>GANAYLNLYKIDIPKKIKRLYFYNPDMEPKLFARNLSRVNNFKFQDSNDLVWIEIPDIDFQITPKNVFQYKVEKEEIIKEEEDKKLFVKTLYKYIKKLFLDNDFYF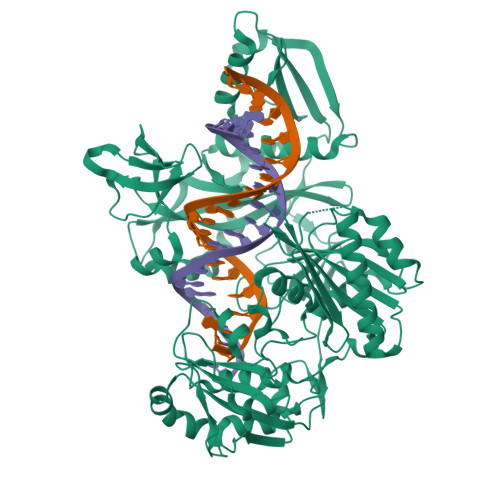KKGNNFISNSEVFSLDSNENVNAHLTYKIKIHNISNEYYLSILPKFTFLSKEPALESAIKSGYLYNIKSGKSFPYISGLDGILKIDIGNNQIVEVAYPENYLFNFTTRDAEKYGFSKEVHEIYKNKVFEGFKKIPKTLGFLNKITNLNENYQLKDGYKIFINVIYKFKNGESRYAKDVFKYSFYKNEQPLKAIFFFSSKKQFFEVQKSLKELFHNKHSVFYRAAAELGFSKVEFLRDSKTKSSAFLYNPEEFTVKNTEFINQIEDNVMAIVLLDKYIGNIDPLVRNFPDNLILQPILKEKLEDIKPFIIKSYVYKMGNFIPECKPFILKKMEDKEKNLYIGIDLSHDTYARKTNLCIAAVDNTGDILYIGKHKNLELNEKMNLDILEKEYIKAFEKYIEKFNVSPENVFILRAGRFIEDIEIIKNFISYNDTKYTLVEVNKNTNINSYDDLKEWIIKLDENTYIYYPKTFLNQKGVEVKILENNTDYTIEEIIEQIYLLTRVAHSTPYTNYKLPYPLHIANKVALTDYEWKLYIPY[2x]>MNHLLSMEHLSTDQIYKLIQKASQFKSGERQLPNFEGKYVANLFFENSTRTKCSFEMAELKL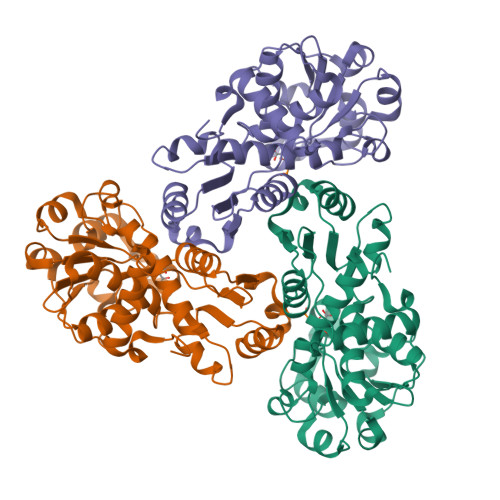GLKTISFETSTSSVSKGESLYDTCKTLESIGCDLLVIRHPFNNYYEKLANINIPIANAGDGSGQHPTQSLLDLMTIYEEYGYFEGLNVLICGDIKNSRVARSNYHSLKALGANVMFNSPNAWIDDSLEAPYVNIDDVIETVDIVMLLRIQHERHGLAEETRFAADDYHQKHGLNEVRYNKLQEHAIVMHPAPVNRGVEIQSDLVEASKSRIFKQMENGVYLRMAVIDELLK[3x]>MVLKSRLEWGEPAFTILDVRDRSTYNDGHIMGAMAMPIEDLVDRASSSLEKSRDIYVYGAGDEQTSQAVNLLRSAGFEHVSELKGGLAAWKAIGGPTELEHHHHHH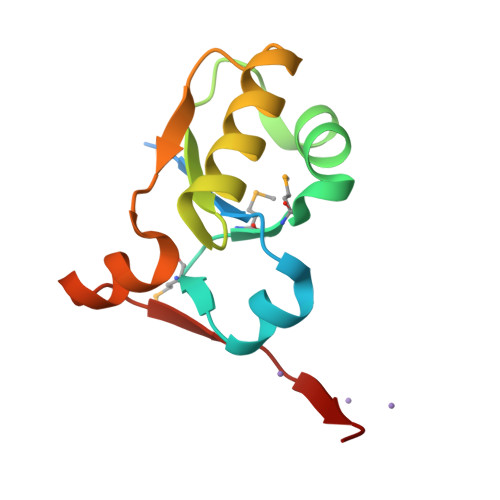[3x]>GAMGNPLRKFKLVFLGEQSVGKTSLITRFMYDSFDNTYQATIGIDFLSKTMYLEDRTVRLQLWDTAGLERFRSLIPSYIRDSTVAVVVYDITNVNSFQQTTKWIDDVRTERGSDVIIMLVGNKTDLADKRQVSIEEGERKAKELNVMFIETSAKAGYNVKQLFRRVAAALPGMESTQDRSREDMIDIKLEK[2x];>GAMEQWCSERLDNQKELMEELYEEKLKILKESLTT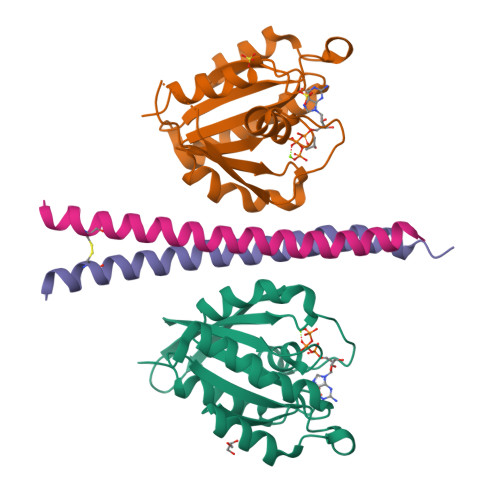FYQEQIQERDEKIEELETLLQEAKQQPAAQQ[2x]>[2x]MADDQGCIEEQGVEDSANEDSVDAKPDRSSFVPSLFSKKKKNVTMRSIKTTRDRVPTYQYNMNFEKLGKCIIINNKNFDKVTGMGVRNGTDKDAEALFKCFRSLGFDVIVYNDCSCAKMQDLLKKASEEDHTNAACFACILLSHGEENVIYGKDGVTPIKDLTAHFRGDRCKTLLEKPKLFFIQACRGTELDDGIQADSGPINDTDANPRYKIPVEADFLFAYSTVPGYYSWRSPGRGSWFVQALCSILEEHGKDLEIMQILTRVNDRVARHFESQSDDPHFHEKKQIPCVVSMLTKELYFSQ

The caspase family of enzymes are responsible for controlling the final steps of inflammation and various cell death pathways. This highly regulated family of endoproteases employ a catalytic cysteine/histidine dyad to hydrolyze peptides with high specificity for aspartate at the P1 position. Initiator caspases (−8, −9) are activated in response to apoptotic stimuli to further activate executioner caspases (−3, −6, −7) by proteolytically cleaving the aspartate‐containing inter‐linker subunit. Once activated, they carry out the final steps of apoptosis by judiciously cleaving hundreds of substrates to dismantle the cell in a controlled fashion.

The current study employed a FBDD approach to identify a series of fragments capable of allosterically inhibiting caspase‐7 (C7). X‐ray crystallography confirmed that these compounds bind at the dimer interface of caspase‐7 more than 17 Å from the active site. The X‐ray crystal structure of caspase‐7 soaked with 1 was determined at a resolution of 2.8 Å. During soaking experiments with 1, electron density appeared in the known allosteric site at the dimer interface of C7 near K160. The carboxyl group in 1 forms an ionic interaction with the neighboring R167, and a hydrogen bond with T163. The binding of 1 occurred more than 5 Å away from C290, the residue utilized for the tethering of thiol‐containing fragments, further supporting the reversibility of the binding of these fragments. The appearance of density in the allosteric site occurred concurrently with the movement of the catalytic cysteine C186 into the P1 substrate‐binding pocket and the disappearance of the active‐site loop density for loops L1, L2, L3, L4, and L2′. Binding of fragment 1 appeared to move E216 towards Y229, displacing it and consequently the L2 loop. The partial occupancy of 0.71 for 1 results in alternate rotamer conformations of E216. Electron density was obtained for only one ligand in each dimer, near one monomer.> ASWSHPQFEKGAMSNYSMSRGHSDKCVGAEDILSEIKEAEKVLNAASDELKREGHNVKTFIDRTSTTQSANLNKIVNWHNANPADVHISVHLNAGKGTGVEVWYYAGDEKGRKLAVEISAKMAKALGLPNRGAKATKDLRFLNSTKGTAVLLEVCFVDRKEDANAIHKSGMYDKLGIAIAEGLTGKTVAAKNPNRHSGAVVDSVPMLSKMDFKSSPIKMYKAGSSLLVYEHNKYWYKAYINDKLCYIYKSFCISNGKKDAKGRIKVRIKSAKDLRIPVWNNTKLNSGKIKWYSPGTK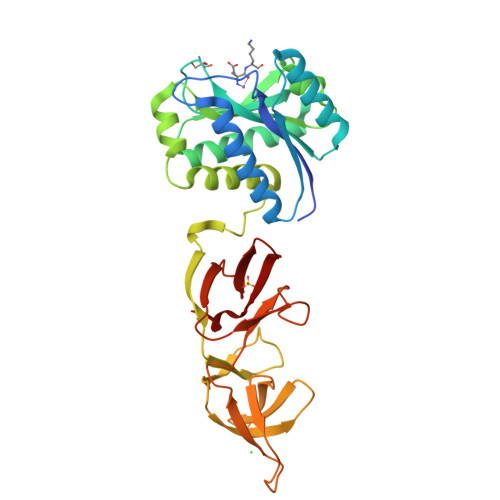LSWYDNKKGYLELWYEKDGWYYTANYFLK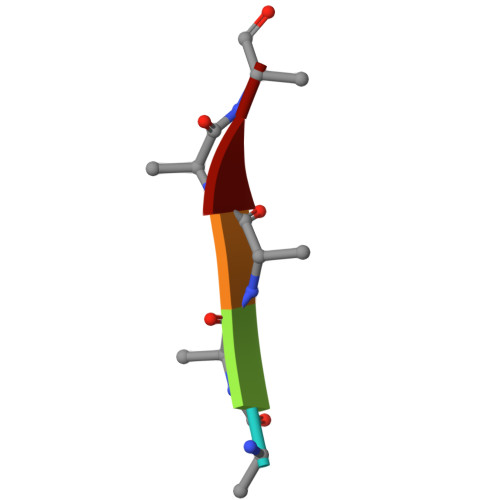> AAAAA>SVDREEMIERFANFLREYTDEDGNPVYRGKITDLLTITPKRSVAIDWMHLNSFDSELAHEVIENPEEGISAAEDAIQIVLREDFQREDVGKIHARFYNLPETLMVKDIGAEHINKLIQVEGIVTRVGEIKPFVSVAVFVCKDCGHEMIVPQKPYESLEKVKKCEQCGSKNIELDVNKSSFVNFQSFRIQDRPETLKGGEMPRFIDGILLDDIVDVALPGDRVIVTGILRVVLEKREKTPIFRKILEVNHIEPVSKEI[6x]

Hexameric MCM rings act as the replicative DNA helicase, encircling the leading strand DNA template at the replication fork. Each Mcm subunit contains three domains. The N-terminal domain (MCMN) possesses an OB (oligonucleotide/oligosaccharide binding)-fold and usually a zinc-binding motif. The MCM complexes of several archaeal organisms consist of six identical subunits and have provided powerful models to investigate the atomic details of MCM structure.

Like SsoMCMN, PfMCMN elutes as a monomer by size-exclusion chromatography (data not shown) but adopts a hexameric arrangement in the crystal structure. The RMSD of the C-subdomain Cα-positions from the sixfold permutation is 3.03 Å and 1.45 Å for hexamers 1 and 2, respectively. In contrast, PfMCMN without DNA bound is highly symmetric and shows minimal RMSD from sixfold symmetry (Figure 1—figure supplements 4–6, RMSD = 0.33 Å), indicating that DNA induces asymmetry in the MCM ring.>ASNFTQFVLVDNGGTGDVTVAPSNFANGVAEWISSNSRSQAYKVTCSVRQSSAQNRKYSIKVEVPKVATQTVGGVELPVAAWRSYLNMELT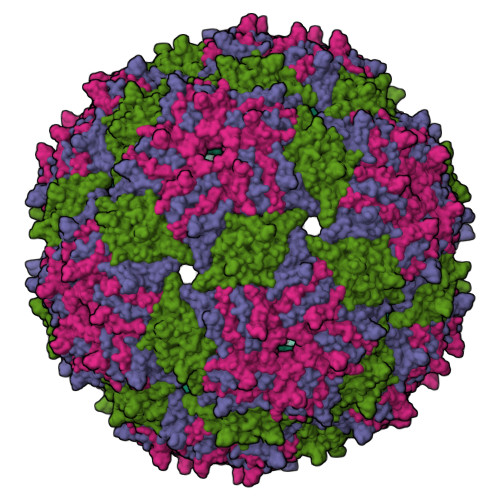IPIFATNSDCELIVKAMQGLLKDGNPIPSAIAANSGIY[3x]> MSKQAAVIELGYMGISVKDPDAWKSFATDMLGLQVLDEGEKDRFYLRMDYWHHRIVVHHNGQDDLEYLGWRVAGKPEFEALGQKLIDAGYKIRICDKVEAQERMVLGLMKTEDPGGNPTEIFWGPRI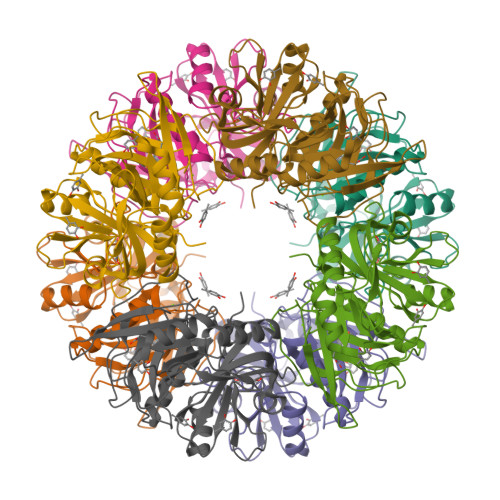DMSNPFHPGRPLHGKFVTGDQGLGHCIVRQTDVAEAHKFYSLLGFRGDVEYRIPLPNGMTAELSFMHCNARDHSIAFGAMPAAKRLNHLMLEYTHMEDLGYTHQQFVKNEIDIALQLGIHANDKALTFYGATPSGWLIEPGWRGATAIDEAEYYVGDIFGHGVEATGYGLDVKLS>MKRSLRKMWRPGEKKEPQGVVYEDVPDDTEDFKESLKVVFEGSAYGLQNFNKQKKLKTCDDMDTFFLHYAAAEGQIELMEKITRDSSLEVLHEMDDYGNTPLHCAVEKNQIESVKFLLSRGANPNLRNFNMMAPLHIAVQGMNNEVMKVLLEHRTIDVNLEGENGNTAVIIACTTNNSEALQILLNKGAKPCKSNKWGCFPIHQAAFSGSKECMEIILRFGEEHGYSRQLHINFMNNGKATPLHLAVQNGDLEMIKMCLDNGAQIDPVEKGRCTAIHFAATQGATEIVKLMISSYSGSVDIVNTTDGCHETMLHRASLFDHHELADYLISVGADINKIDSEGRSPLILATASASWNIVNLLLSKGAQVDIKDNFGRNFLHLTVQQPYGLKNLRPEFMQMQQIKELVMDEDNDGCTPLHYACRQGGPGSVNNLLGFNVSIHSKSKDKKSPLHFAASYGRINTCQRLLQDISDTRLLNEGDLHGMTPLHLAAKNGHDKVVQLLLKKGALFLSDHNGWTALHHASMGGYTQTMKVILDTNLKCTDRLDEDGNTALHFAAREGHAKAVALLLSHNADIVLNKQQASFLHLALHNKRKEVVLTIIRSKRWDECLKIFSHNSPGNKCPITEMIEYLPECMKVLLDFCMLHSTEDKSCRDYY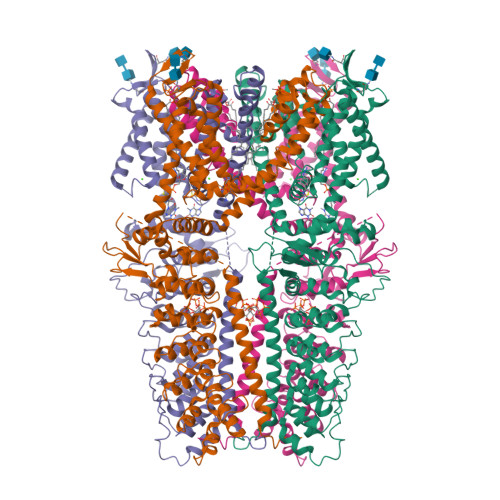IEYNFKYLQCPLEFTKKTPTQDVIYEPLTALNAMVQNNRIELLNHPVCKEYLLMKWLAYGFRAHMMNLGSYCLGLIPMTILVVNIKPGMAFNSTGIINETSDHSEILDTTNSYLIKTCMILVFLSSIFGYCKEAGQIFQQKRNYFMDISNVLEWIIYTTGIIFVLPLFVEIPAHLQWQCGAIAVYFYWMNFLLYLQRFENCGIFIVMLEVILKTLLRSTVVFIFLLLAFGLSFYILLNLQDPFSSPLLSIIQTFSMMLGDINYRESFLEPYLRNELAHPVLSFAQLVSFTIFVPIVLMNLLIGLAVGDIAEVQKHASLKRIAMQVELHTSLEKKLPLWFLRKVDQKSTIVYPNKPRSGGMLFHIFCFLFCTGEIRQEIPNADKSLEMEILKQKYRLKDLTFLLEKQHELIKLIIQKMEIISETEDDDSHCSFQDRFKKEQMEQRNSRWNTVLRAVKAKTHHLEPAENLYFQ[4x]>[4x]MDKQYPVRQWAHGADLVVSQLEAQGVRQVFGIPGAKIDKVFDSLLDSSIRIIPVRHEANAAFMAAAVGRITGKAGVALVTSGPGCSNLITGMATANSEGDPVVALGGAVKRADKAKQVHQSMDTVAMFSPVTKYAIEVTAPDALAEVVSNAFRAAEQGRPGSAFVSLPQDVVDGPVSGKVLPASGAPQMGAAPDDAIDQVAKLIAQAKNPIFLLGLMASQPENSKALRRLLETSHIPVTSTYQAAGAVNQDNFSRFAGRVGLFNNQAGDRLLQLADLVICIGYSPVEYEPAMWNSGNATLVHIDVLPAYEERNYTPDVELVGDIAGTLNKLAQNIDHRLVLSPQAAEILRDRQHQRELLDRRGAQLNQFALHPLRIVRAMQDIVNSDVTLTVDMGSFHIWIARYLYTFRARQVMISNGQQTMGVALPWAIGAWLVNPERKVVSVS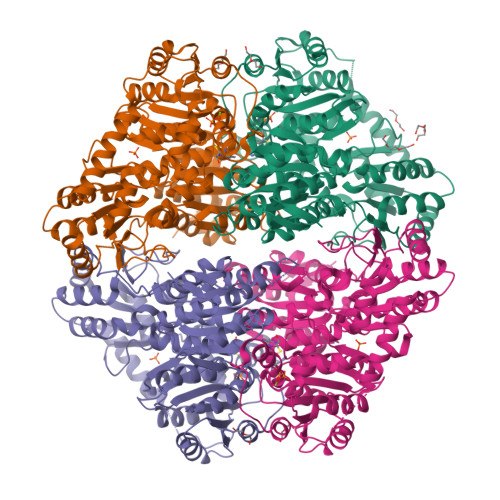GDGGFLQSSMELETAVRLKANVLHLIWVDNGYNMVAIQEEKKYQRLSGVEFGPMDFKAYAESFGAKGFAVESAEALEPTLRAAMDVDGPAVVAIPVDYRDNPLLMGQLHLSQILEHHHHHH> MRSIARRTAVGAALLLVMPVAVWISGWRWQPGEQSWLLKAAFWVTETVTQPWGVITHLILFGWFLWCLRFRIKAAFVLFAI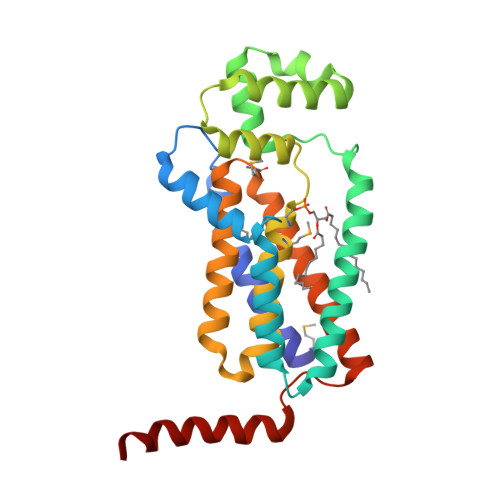LAAAILVGQGVKSWIKDKVQEPRPFVIWLEKTHHIPVDEFYTLKRAERGNLVKEQLAEEKNIPQYLRSHWQKETGFAFPSGHTMFAASWALLAVGLLWPRRRTLTIAILLVWATGVMGSRLLLGMHWPRDLVVATLISWALVAVATWLAQRICGPLTPPAEENREIAQREQESLEHHH> SGGGDGSTYSA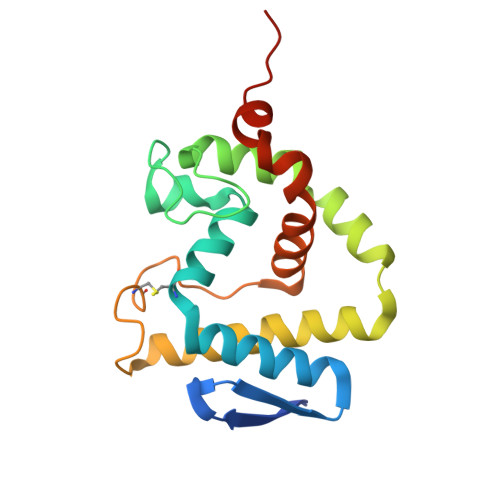EIRRTTMGVPHIKAGNWGSAGYGFGYVQAQDNLCTMADSFLTYRGERSRHLGGSAQLVYNSTLGRPRNIDSDFFHRHVISDEAVDRTMAAQPAKLLQMVEGFAAGYNRYVREAKAGGSAHAACRSEAWVQPITARDVWRRIYAANLAGGYSNFAEAIANAQPPQAKA> DKATIPSESPFAA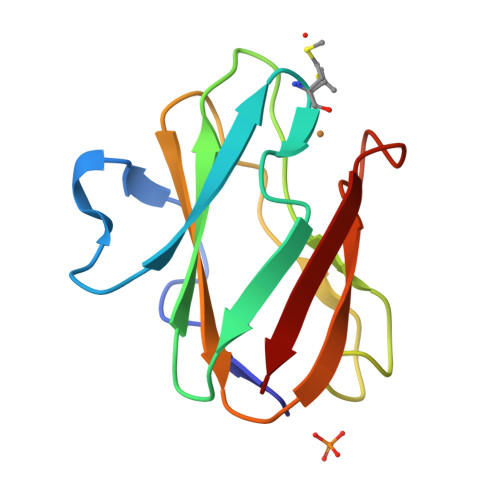AEVADGAIVVDIAKMKYETPELHVKVGDTVTWINREAAPHNVHFVAGVLGEAALKGPMMKKEQAYSLTFTEAGTYDYHCTPHPFMRGKVVVE> RGEADLFDSGDIFST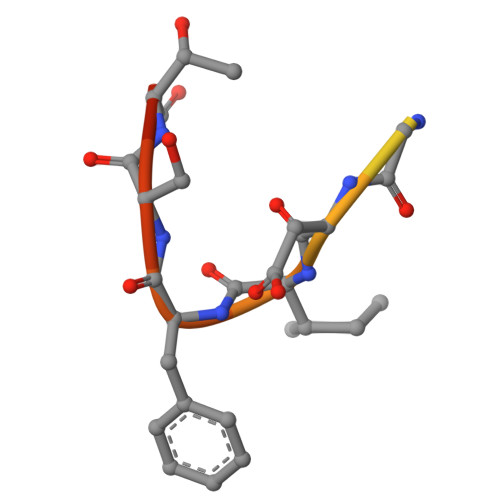GT> SNADDLQMIEMHELIQEFYYYALTKTVEGEQALTYLQERGFTDALIKERGIG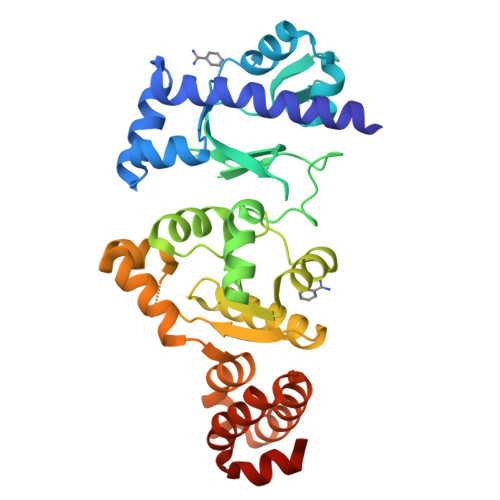FAPDSSHFCHDFLQKKGYDIELAYEAGLLSRNEENFSYYDRFRNRIMFPLKNAQGRIVGYSGRTYTGQEPKYLNSPETPIFQKRKLLYNLDKARKSIRKLDEIVLLEGFMDVIKSDTAGLKNVVATMGTQLSDEHITFIRKLTSNITLMFDGDFAGSEATLKTGQHLLQQGLNVFVIQLPSGMDPDEYIGKYGNDAFTTFVKNDKKSFAHYKVSILKDEIAHNDLSYERYLKELSHDISLMKSSILQQKAINDVAPFFNVSPEQLANEIQFNQAPAN> GPKDEERRESRIQSYSPQAFKFFMEQHVENVLKSHQQRLHRKKQLENEMMRVG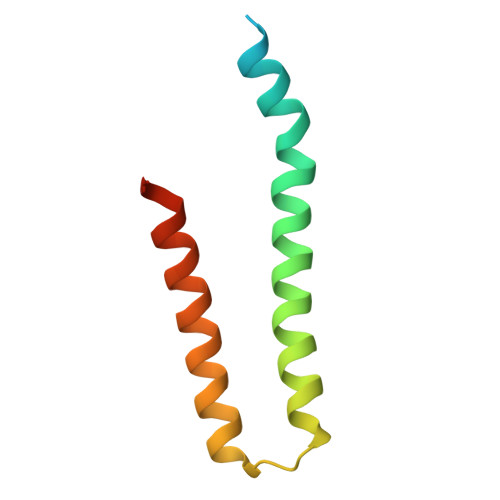LSQDAQDQMRKMLCQKESNYIRLKRAKMDKSM> AETV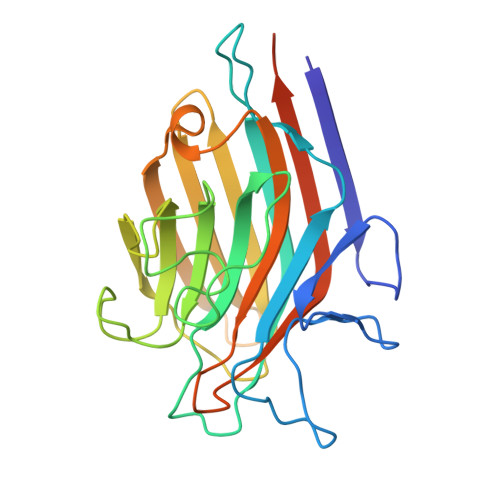SFSWNKFVPKQPNMILQGDAIVTSSGKLQLNKVDENGTPKPSSLGRALYSTPIHIWDKETGSVASFAASFNFTFYAPDTKRLADGLAFFLAPIDTKPQTHAGYLGLFNENESGDQVVAVEFDTFRNSWDPPNPHIGINVNSIRSIKTTSWDLANNKVAKVLITYDASTSLLVASLVYPSQRTSNILSDVVDLKTSLPEWVRIGFSAATGLDIPGESHDVLSWSFASNLPHASSNIDPLDLTSFVLHEAI> MMLSLNNLQNIIYNPVIPFVGTIPDQLDPGTLIVIRGHVPSDADRFQVDLQNGSSVKPRADVAFHFNPRFKRAGCIVCNTLINEKWGREEITYDTPFKREKSFEIVIMVLKDKFQVAVNGKHTL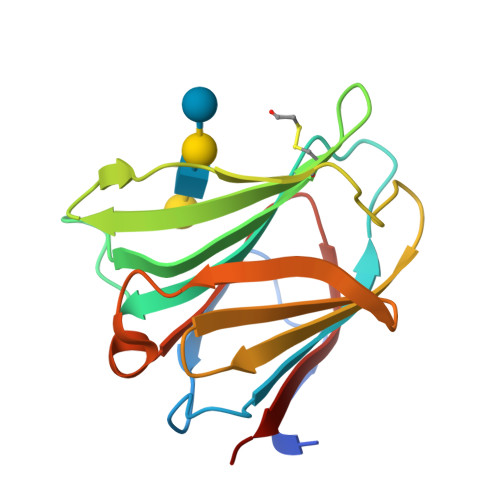LYGHRIGPEKIDTLGIYGKVNIHSIGFSFSS>MERKQKNSLFNYIYSLMDVRGKFLFFSMLFITSLSSIIISISPLILAKITDLLSGSLSNFSYEYLVLLACLYMFCVISNKASVFLFMILQSSLRINMQKKMSLKYLRELYNENITNLSKNNAGYTTQSLNQASNDIYILVRNVSQNILSPVIQLISTIVVVLSTKDWFSAGVFFLYILVFVIFNTRLTGSLASLRKHSMDITLNSYSLLSDTVDNMIAAKKNNALRLISERYEDALTQENNAQKKYWLLSSKVLLLNSLLAVILFGSVFIYNILGVLNGVVSIGHFIMITSYIILLSTPVENIGALLSEIRQSMSSLAGFIQRHAENKATSPSIPFLNMERKLNLSIRELSFSYSDDKKILNSVSLDLFTGKMYSLTGPSGSGKSTLVKIISGYYKNYFGDIYLNDISLRNISDEDLNDAIYYLTQDDYIFMDTLRFNLRLANYDASENEIFKVLKLANLSVVNNEPVSLDTHLINRGNNYSGGQKQRISLARLFLRKPAIIIIDEATSALDYINESEILSSIRTHFPDALIINISHRINLLECSDCVYV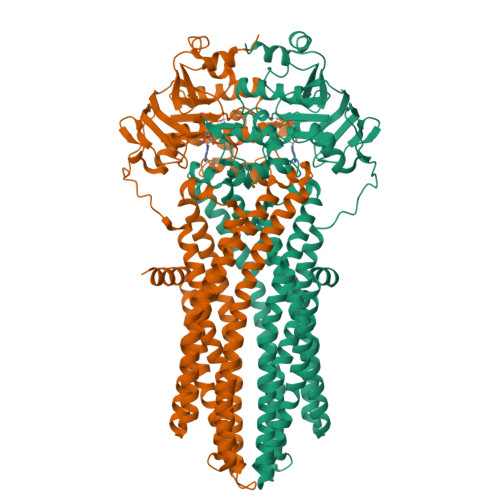LNEGNIVASGHFRDLMVSNEYISGLASVTE[2x]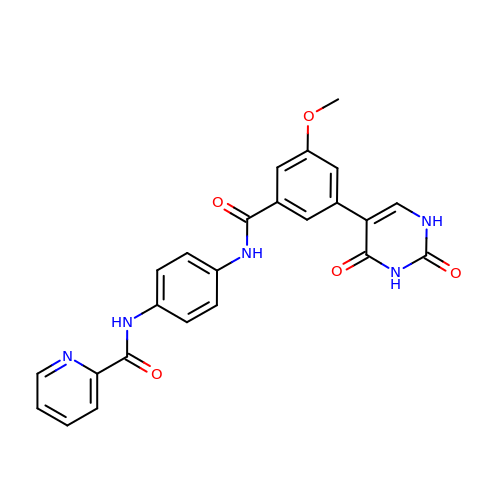N-(4-{[3-(2,4-dioxo-1,2,3,4-tetrahydropyrimidin-5-yl)-5-methoxybenzoyl]amino}phenyl)pyridine-2-carboxamide | C24 H19 N5 O5 | IDGYBMGDEPAAQL-UHFFFAOYSA-N>MALFFRTRDRPLRPGDPYPLGSNWIEDDDGVNFSLFSENAEKVELLLYSLTNQKYPKEIIEVKNKTGDIWHVFVPGLRPGQLYAYRVYGPYKPELGLRFNPNKVLIDPYAKAINGSVIWNDAVFGYKIGDQNQDLTYDERDSGEYVPKSVVINPYFEWDDEDFIKGKKVPLKDTVIYEVHVKGFTKLRLDLPENIRGTYEGLASEQMISYLKDLGITTVELMPVFHFIDQRFLTDKGLTNYWGYDPINFFSPECRYSSTGCLGGQVLSFKKMVNELHNAGIEVIIDVVYNHTAEGNHLGPTLSFRGIDNTAYYMLQPDNKRYYLDFTGTGNTLNLSHPRVIQMVLDSLRYWVTEMHVDGFRFDLAAALARELYSVNMLNTFFIALQQDPILSQVKLIAEPWDVGQGGYQVGNFPYQWAEWNGKYRDSIRRFWRGEALPYSEIANRLLGSPDIYLGNNKTPFASINYVTSHDGFTLEDLVSYNQKHNEANGFNNQDGMNENYSWNCGAEGPTNDQNVVICREKQKRNFMITLLVSQGTPMILGGDELSRTQRGNN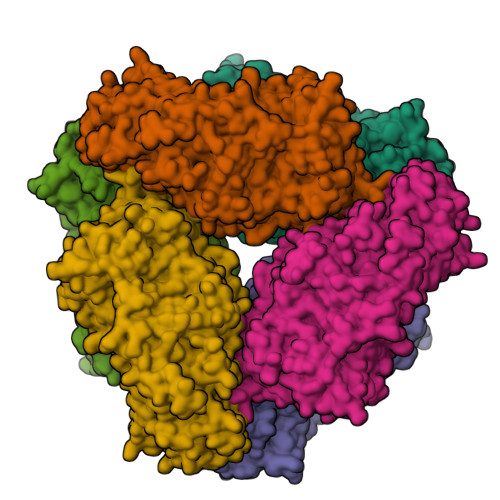NAFCQDNEITWFDWNLDERKSKFLEFVKKMIQFYRAHPAFRRERYFQGKKLFGMPLKDVTFYTLEGREVDEKTWSSPTQLVIFVLEGSVMDEINMYGERIADDSFLIILNANPNNVKVKFPKGKWELVISSYLREIKPEERIIEGEKELEIEGRTALVYRRIEL[2x]>GSSGSSGSALDQLKQFTTVVADTGDFNAIDEYKPQDATTNPSLILAAAQMPAYQELVEEAIAYGKKLGGPQEEQIKNAIDKLFVLFGAEILKKIPGRVSTEVDARLSFDKDAMVARARRLIELYKEAGVGKDRILIKLSSTWEGIQAGKELEEQHGIHCNMTLLFSFAQAVACAEAGVTLISPFV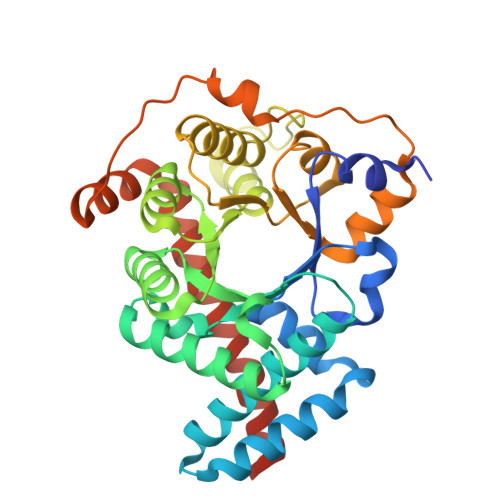GRILDWHVANTDKKSYEPQGDPGVKSVTKIYNYYKKFGYKTIVMGASFRNTGEIKALAGCDFLTISPKLLGELLKDNSKLAPALSVKAAQTSDSEKIHLDEKAFRWLHNEDQMAVEKLSDGIRKFAADAIKLERMLTERMFSAENGK[2x]>[2x]SDKIIHVTDD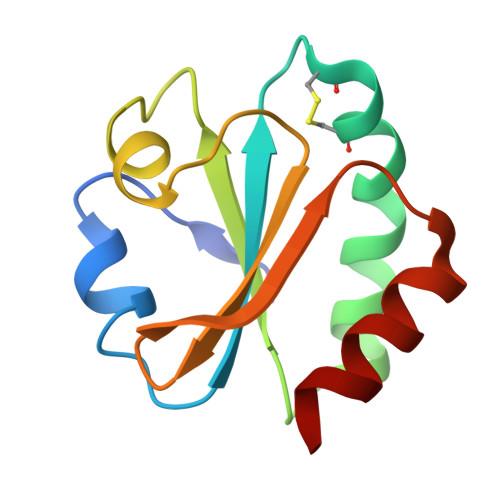SFDTDVLKADGAILVDFWAEWCGPCKMIAPILDEIADEYQGKLTVAKLNIDQNPGTAPKYGIRGIPTLLLFKNGEVAATKVGALSKGQLKEFLDANLA> NDPGKMLKDAIDKQAAGALVA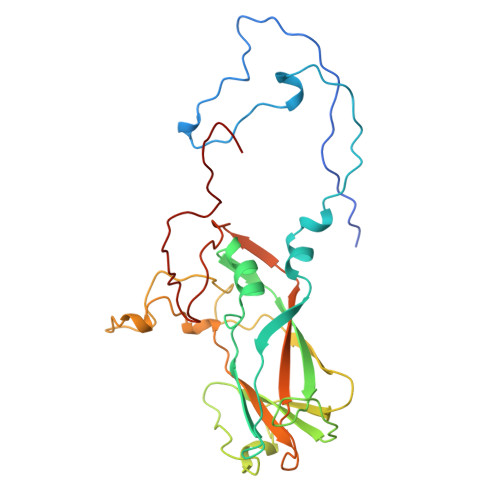GTSTSTHSVATDSTPALQAAETGATSTARDESMIETRTIVPTHGIHETSVESFFGRSSLVGMPLLATGTSITHWRIDFREFVQLRAKMSWFTYMRFDVEFTIIATSSTGQNVTTEQHTTYQVMYVPPGAPVPSNQDSFQWQSGCNPSVFADTDGPPAQFSVPFMSSANAYSTVYDGYARFMDTDPDRYGILPSNFLGFMYFRTLEDAAHQVRFRIYAKIKHTSCWIPRAPRQAPYKKRYNLVFSGDSDRICSNRASLTSY>[2x]DEITKKYIKDNIINVDD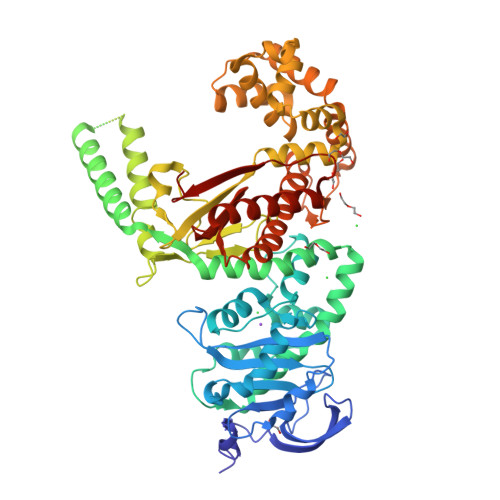NIIKKKDIFKLKNENNEITECAFEYFESKKKFDDDIESRFFIINDNNYNENINLIYKDIKYCGLNIQTTGLEVFDENIRLIQIAVENYPVIIYDMFNINKKDILDGLRKVLENKNIIKIIQNGKFDAKFLLHNNFKIENIFDTYIASKLLDKNKNMYGFKLNNIVEKYLNVILDKQQQNSVWNNSLLNNNQLFYAARDSSCLLKLYKKLKEEIKKENLHIVNDIENKCILPICDMELNGIKVDLENLQKSTNEILNELNIEKDNLKKKLKDENINVNSQQQVLKALQKNNVRDISNKLIENTSDSNLKNFLNHEEIISLRNYRRLYKLYSAFYLKLPLHINTKTNKIHTTFNQLKTFSGRFSSEKPNLQQIPRQKNIREIFIPNDNNIFIIADFKQIELKIAAEITNDEIMLKAYNNNIDLHTLTASIITKKNIPDINKEDRHIAKAINFGLIYGMNYVNLKNYANTYYGLNMSLDQCLYFYNSFFEHYKGIYKWHNQVKQKRALQYSTLSNRKVIFPYFSFTKALNYPVQGTCADILKLALVDLYDNLKDINGKIILCVHDEIIIEVNKKFQEEALKILVQSMENSASYFLKKVKCEVSVKIAENWGSKD> MIRLYPEQLRAQLNEGLRAAYLLLGNDPLLLQESQDAVRQVAAAQGFEEHHTFSIDPNTDWNAIFSLCQAMSLFASRQTLLLLLPENGPNAAINEQLLTLTGLLHDDLLLIVRGNKLSKAQENAAWFTALANRSVQVTCQTPEQAQLPRWVAARAKQLNLELDDAANQVLCYCYEGNLLALAQALERLSLLWPDGKLTLPRVEQAVNDAAHFTPFHWVDALLMGKSKRALHILQQLRLEGSEPVILLRTLQRELLLLVNLKRQSAHTPLRALFDKHRVWQNRRGMMGEALNRLSQTQLRQAVQLLTRTELTLKQDYGQSVWAELEGLSLLLCHKPLADVFIDG;>GPHMSYQVLARKWRPQTFADVVGQEHVLTALANGLSLGRIHHAYLFSGTRGVGKTSIARLLAKGLNCETGITATPCGVCDNCREIEQGRFVDLIEIDAASRTKVEDTRDLLDNVQYAPARGRFKVYLIDEVHMLSRHSFNALLKTLEEPPEHVKFLLATTDPQKLPVTILSRCLQFHLKALDVEQIRHQLEHILNEEHIAHEPRALQLLARAAEGSLRDALSLTDQAIASGDGQVSTQAVSAMLGTLDDDQALSLVEAMVEANGERVMALINEAAARGIEWEALLVEMLGLLHRIAMVQLSPAALGNDMAAIELRMRELARTIPPTDIQLYYQTLLIGRKELPYAPDRRMGVEMTLLRALAFHPRMPLPEPEVPRQ[3x];> GPHMRWYPWLRPDFEKLVASYQAGRGHHALLIQALPGMGDDALIYALSRYLLCQQPQGHKSCGHCRGCQLMQAGTHPDYYTLAPEKGKNTLGVDAVREVTEKLNEHARLGGAKVVWVTDAALLTDAAANALLKTLEEPPAETWFFLATREPERLLATLRSRCRLHYLAPPPEQYAVTWLSREVTMSQDALLAALRLSAGSPGAALALFQGDNWQARETLCQALAYSVPSGDWYSLLAALNHEQAPARLHWLATLLMDALKRHHGAAQVTNVDVPGLVAELANHLSPSRLQAILGDVCHIREQLMSVTGINRELLITDLLLRIEHYLQPGVVLPVPHL;>GPHMKFTVEREHLLKPLQQVSGPLGGRPTLPILGNLLLQVADGTLSLTGTDLEMEMVARVALVQPHEPGATTVPARKFFDICRGLPEGAEIAVQLEGERMLVRSGRSRFSLSTLPAADFPNLDDWQSEVEFTLPQATMKRLIEATQFSMAHQDVRYYLNGMLFETEGEELRTVATDGHRLAVCSMPIGQSLPSHSVIVPRKGVIELMRMLDGGDNPLRVQIGSNNIRAHVGDFIFTSKLVDGRFPDYRRVLPKNPDKHLEAGCDLLKQAFARAAILSNEKFRGVRLYVSENQLKITANNPEQEEAEEILDVTYSGAEMEIGFNVSYVLDVLNALKCENVRMMLTDSVSSVQIEDAASQSAAYVVMPMRL[2x]

Clamp loaders are pentameric ATPases that place circular sliding clamps onto DNA, where they function in DNA replication and genome integrity. Because the sliding clamp is a closed ring in solution, it needs to be opened and placed onto DNA by a separate ATPase complex called the clamp loader. All clamp loaders are pentameric ATPases of the AAA + family (ATPases associated with various cellular activities). Here we describe a series of structures of the E. coli clamp loader in the process of placing the clamp onto a p/t-junction.

A surprising class of DNA-primed particles exhibits an open clamp structure, but the collar region is in a different conformation from all other γ-complex structures reported herein or elsewhere. The collar region of the B subunit shifts upward away from the AAA+ spiral. The collar regions of the C, D, and E subunits are static, and the A subunit only moves slightly. The movement of the collar opens a large pore between the A and B subunits. Moreover, this movement alters the center of the collar at the binding site for the ψ protein, an accessory factor that, together with the χ protein, acts as an adaptor linking the clamp loader to the single-stranded binding protein (SSB). The Altered-Collar state shifts the binding site such that it is incompatible with the known binding pose of the ψ protein. We attribute this structure to an off- or parallel-pathway intermediate and discuss potential implications for the Altered-Collar conformational changes in the Discussion. The Altered-Collar state observed here severely disrupts the ψ protein binding site, suggesting that this conformation is incompatible with ψ protein binding. It is possible that the Altered-Collar state functions as a means for disengaging the clamp loader’s linkage to SSB through the ψ protein. Because the E. coli clamp loader can readily load ß-clamp onto nicked DNA, we speculate that this pore could function as a channel for the unwound primer strand of nicked DNA to exit the central chamber, similar to RFC.>[2x]GSHMASMTGGQQMGRGSAAQRQGALA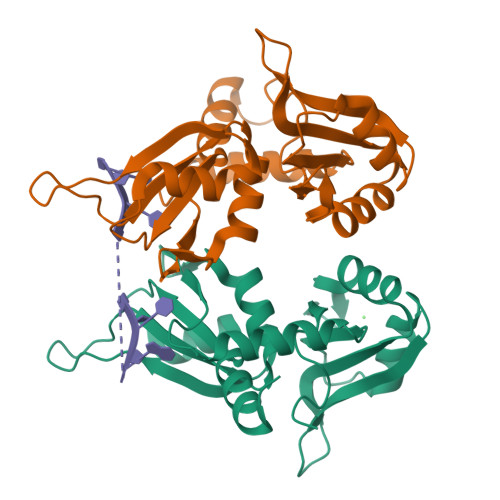IMSRVYVGSIYYELGEDTIRQAFAPFGPIKSIDMSWDSVTMKHKGFAFVEYEVPEAAQLALEQMNSVMLGGRNIKVGRPSNIGQAQPIIDQLAEEARAFNRIYVASVHQDLSDDDIKSVFEAFGKIKSATLARDPTTGKHKGYGFIEYEKAQSSQDAVSSMNLFDLGGQYLRVGKAVTPPMPLLTPATPG> AQSVPYGVSQIKAPALHSQGYCGSNVKVAVIDSGIDSSHPDLKVAGGASFVPSETNPFQDNNSHGTHVAGTVAALNNSIGVLGVAPCASLYAVKVLGADGSGQYSWIINGIEWAIANNMDVINMSLGGPSGSAALKAAVDKAVASGV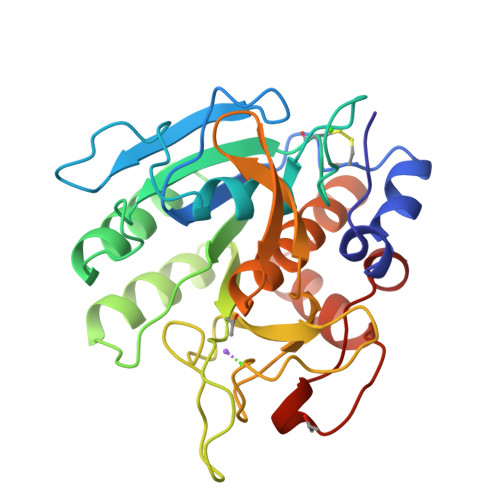VVVAAAGNEGTSGSSSTVGYPAKYPSVIAVGAVDSSNQRASFSSVGPELDVMAPGVSIQSTLPGNKYGAKSGTSMASPHVAGAAALILSKHPNWTNTQVRSSLENTTTKLGDSFYYGKGLINVQAAAQ>MAKDKEFQVLFVLTILTLISGTIFYSTVEGLRPIDALYFSVVTLTTVGYGDFSPQTDFGKIFTILYIFIGIGLVFGF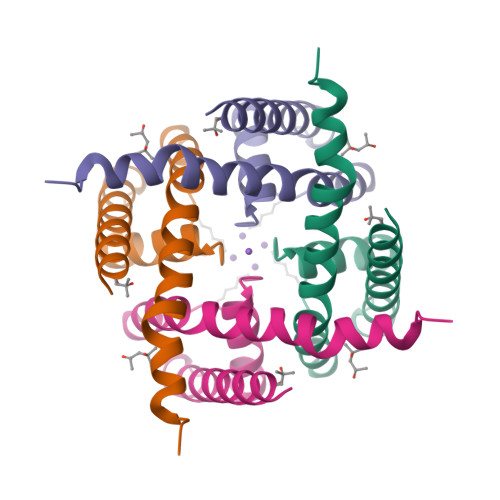IHKLAVNVQLPSILSNLVPR[2x]>[2x]MTGDHIKVIYFNGRGRAESIRMTLVAAGVNYEDERISFQDWPKIKPTIPGGRLPAVKITDNHGHVKWMVESLAIARYMAKKHHMMGGTEEEYYNVEKLIGQAEDLEHEYY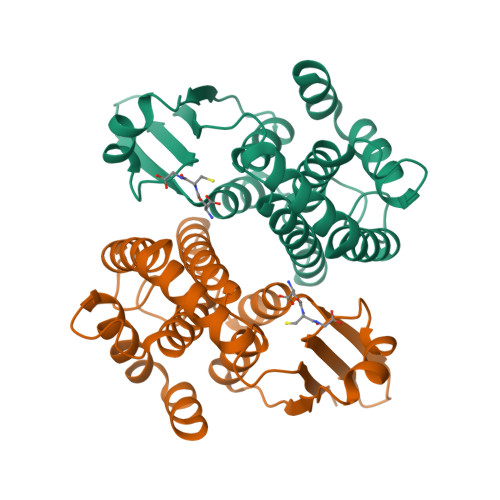KTLMKPEEEKQKIIKEILNGKVPVLLDIICESLKASTGKLAVGDKVTLADLVLIAVIDHVTDLDKEFLTGKYPEIHKHRENLLASSPRLAKYLSDRAATPF>SNAMTQFAFVFPGQGSQSVGMLAEMAANYPIVEETFAEASAALGYDLWALTQQGPAEELNKTWQTQPALLTASVALWRVWQQQGGKMPALMAGHSLGEYSALVCAGVINFADAVRLVEMRGKFMQEAVPEGTGGMSAIIGLDDASIAKACEESAEGQVVSPVNFNSPGQVVIAGHKEAVERAGAACKAAGAKRALP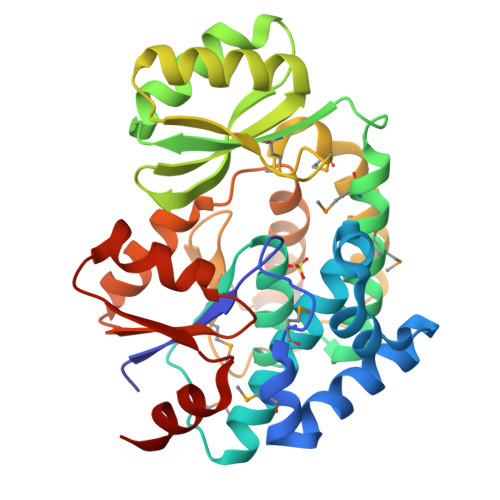LPVSVPSHCALMKPAADKLAVELAKITFSAPTVPVVNNVDVKCETDAAAIRDALVRQLYNPVQWTKSVEFIAAQGVEHLYEVGPGKVLTGLTKRIVDTLTASALNEPAALSAALTQ[2x]> MSKSIYEQYLQAKADNPGKYARDLATLMGISEAELTHSRVSHDAK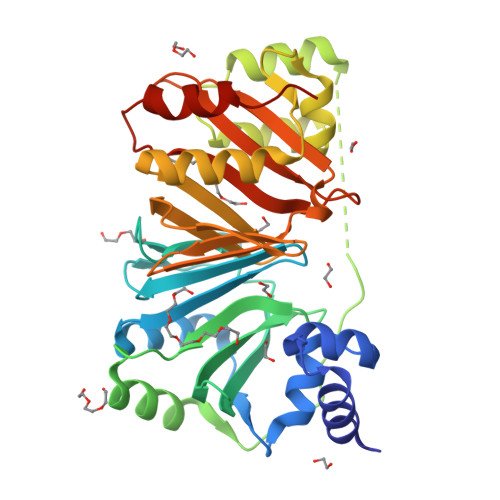RLKGDARALLAALEAVGEVKAITRNTYAVHEQMGRYENQHLNGHAGLILNPRNLDLRLFLNQWASAFTLTEETRHGVRHSIQFFDHQGDALHKVYVTEQTDMPAWEALLAQFITTENPELQLEPLSAPEVTEPTATDEAVDAEWRAMTDVHQFFQLLKRNNLTRQQAFRAVGNDLAYQVDNSSLTQLLNIAQQEQNEIMIFVGNRGCVQIFTGMIEKVTPHQDWINVFNQRFTLHLIETTIAESWITRKPTKDGFVTSLELFAADGTQIAQLYGQRTEGQPEQTQWRDQIARLNNKDIAA>GSSGSSGSSSGKPGPTVIKVQNMPFTVSIDEILDFFYGYQVIPGSVCLKYNEKGMPTGEAMVAFESRDEATAA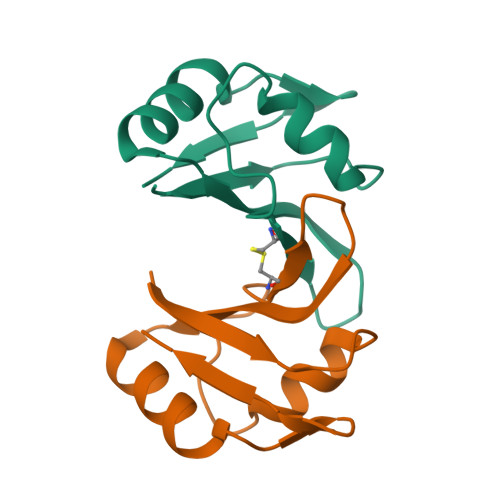VIDLNDRPIGSRKVKLSGPSSG[4x]>MRGSHHHHHHGSMVLGKPQTDPTLEWFLSHCHIHKYPSKSTLIHQGEKAETLYYIVKGSVAVLIKDEEGKEMILSYLNQGDFIGELGLFEEGQERSAWVRAKTACEVAEISYKKFRQLIQVNPDILMRLSAQMARRLQVTSEKVGNLAFLDVTGRIAQTLLNLAKQPDAMTHPDGMQIKITRQEIGQIVGCS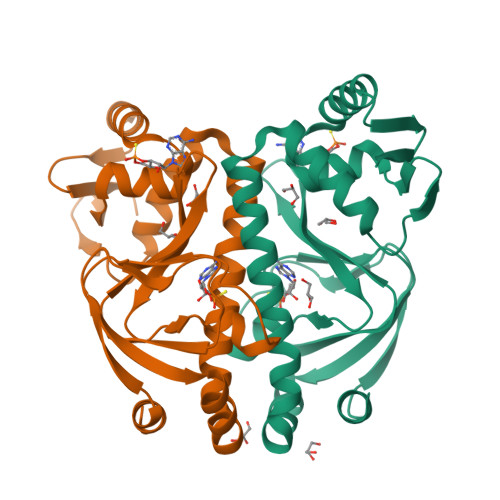RETVGRILKMLEDQNLISAHGKTIVVYGTR[2x]>GSAENESTPIQQLLEHFLRQLQRKDPHGFFAFPVTDAIAPGYSMIIKHPMDFGTMKDKIVANEYKSVTE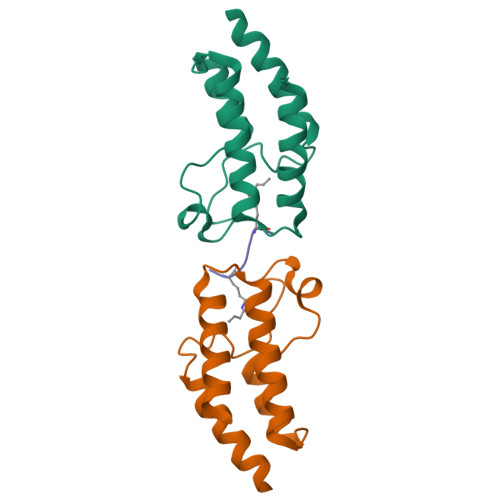FKADFKLMCDNAMTYNRPDTVYYKLAKKILHAGFKMMSK[4x];>SGRGXGGXGLG[2x]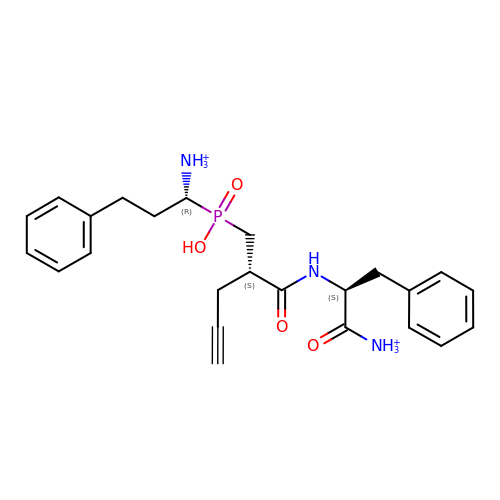[(1~{R})-1-[[(2~{S})-2-[[(2~{S})-1-azaniumyl-1-oxidanylidene-3-phenyl-propan-2-yl]carbamoyl]pent-4-ynyl]-oxidanyl-phosphoryl]-3-phenyl-propyl]azanium | C24 H32 N3 O4 P | QCPJTEUURKCRNT-BHIFYINESA-P> GPGYQDPARSVRHIAIPAHRGLITDRNGEPLAVSTPVTTLWANPKELMTAKERWPQLAAALGQDTKLFADRIEQNAEREFIYLVRGLTPEQGEGVIALKVPGVYSIEEFRRFYPAGEVVAHAVGFTDVDDRGREGIELAFDEWLAGVPGKRQVLKDRRGRVIKDVQVTKNAKPGKTLALSIDLRLQYLAHRELRNALLENGAKAGSLVIMDVKTGEILAMTNQPTYNPNNRRNLQPAAMRNRAMIDVFEPGSTVKPFSMSAALASGRWKPSDIVDVYPGTLQIGRYTIRDVSRNSRQLDLTGILIKSSNVGISKIAFDIGAESIYSVMQQVGLGQDTGLGFPGERVGNLPNHRKWPKAETATLAYGYGLSVTAIQLAHAYAALANDGKSVPLSMTRVDRVPDGVQVISPEVASTVQGMLQQVVEAQGGVFRAQVPGYHAAGKSGTARKVSVGTKGYRENAYRSLFAGFAPATDPRIAMVVVIDEPSKAGYFGGLVSAPVFSKVMAGALRLMNVPPDNLPTATEQQQVNAAP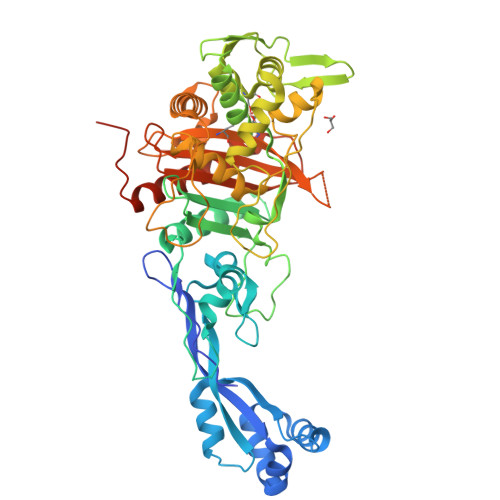AKGGRG>[2x]MDWPHAGRPAHELRYSIYRDLWERGFFLSAAGKFGGDFLVYPGDPLRFHAHYIAQCW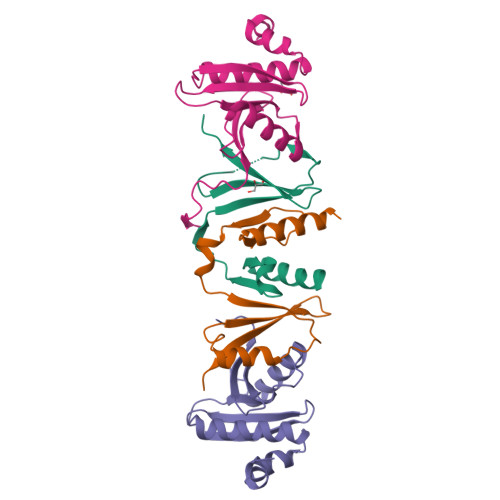APEDTIPLQDLVAAGRLGTSVRKTLLLCSPQPDGKVVYTSLQWASLQ;>MGHHHHHHHHHHGENLYFQGFGDGGGAPSWAPEDAWMGTHPKYLEMMELDIGDATQVYVAFLVYLDLMESKSWHEVNCVGLPELQLICLVGTEIEGEGLQTVVPTPITASLSHNRIREILKASRKLQGDPDLPMSFTLAIVESDSTIVYYKLTDGFMLPDPQNISLR[2x]> HAKPPYSYISLITM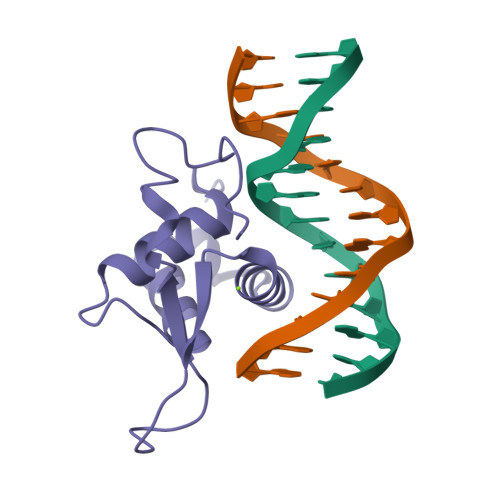AIQQAPGKMLTLSEIYQWIMDLFPYYRENQQRWQNSIRHSLSFNDCFVKVARSPDKPGKGSYWALHPSSGNMFENGCYLRRQKRFKLA> ARRPSVIWLSFQECTGCTESLTRAHAPTLEDLILDFISLDYHHTLQAASGEAAEAARLQAMDENRGQYLVIVDGSIPGPDANPGFSTVAGHSNYSILMETVEHAAAVIAVGTCAAFGGLPQARPNPTGAMSVMDLVRDKPVINVPGCPPIPMVITGVIAHYLVFGRLPELDGYGRPLAFYGQSIHDRCYRRPFY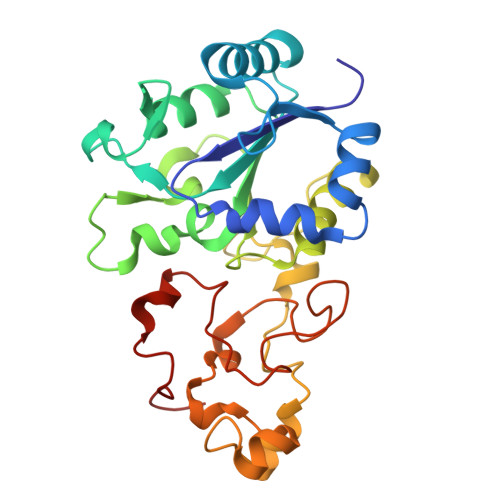DKGLFAESFDDEGAKQGWCLYRLGCKGPTTYNACATMKWNDGTSWPVEAGHPCLGCSEPQFWDAGGFYEPVSVPL> GSMSEQSICQARAAVM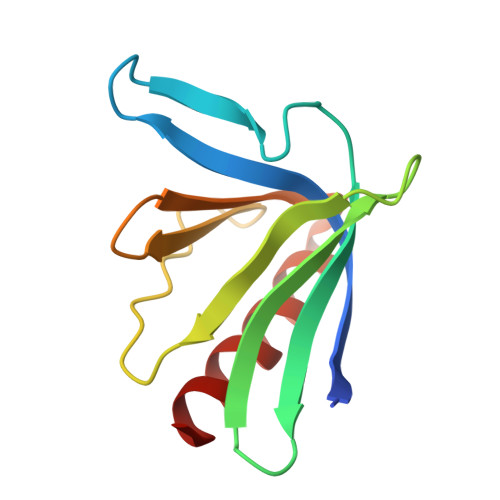VYDDANKKWVPAGGSTGFSRVHIYHHTGNNTFRVVGRKIQDHQVVINCAIPKGLKYNQATQTFHQWRDARQVYGLNFGSKEDANVFASAMMHALEVL> MKRIKCNKVRTVTEIVNSDEKIQKTYELAEFDLKNLSSLESYETLKIKLALSKYMAMLSTLEMTQPLLEIFRNKADTRQIAAVVFSTLAFIHNRFHPLVTNFTNKMEFVVTETNDTSIPGEPILFTENEGVLLCSVDRPSIVKMLSREFDTEALVNFENDNCNVRIAKTFGASKRKNTTRSDDYESNKQPNYDMDLSDFSITEVEATQYLTLLLTVEHAYLHYYIFKNYGVFEYCKSLTDHSLFTNKLRSTMSTKTSNLLLSKFKFTIEDFD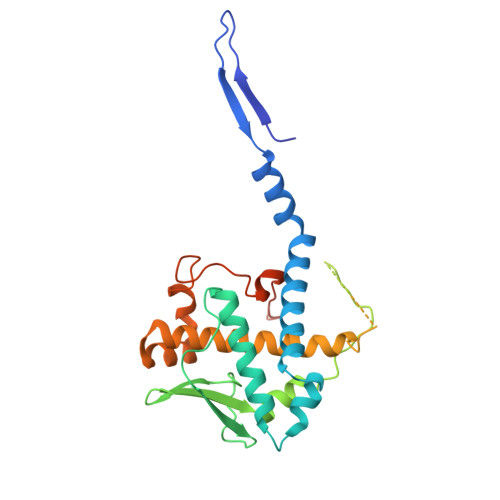KINSNSVTSGFNIYNFNK> MNYNLSKYPDDVSRLFKPRPPLSYKRPTDYPYAKRQTNPNITGVANLLSTSLKHYMEEFPEGSPNNHLQRYEDIKLSKIKNAQLLDRRLQNWNPNVDPHIKDTDPYRTIFIGRLPYDLDEIELQKYFVKFGEIEKIRIVKDKITQKSKGYAFIVFKDPISSKMAFKEIGVHRGIQIKDRICIVDIERGRTVKYFKPRRLGGGLGGRGYSNRDSRLPGRFASASTSNPAERNYAPRLPRRETSSSAYSADRYGSSTLDARYRGNRPLLSAATPTAAVTSVYKSRNS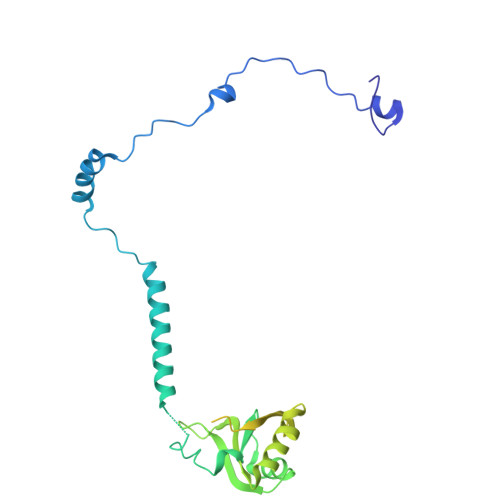RTRESQPAPKEAPDY> KKQDPPVTHDLRVSLEEIYSGCTKKMKISHKRLNPDGKSIRNEDKILTIEVKKGWKEGTKITFPKEGDQTSNNIPADIV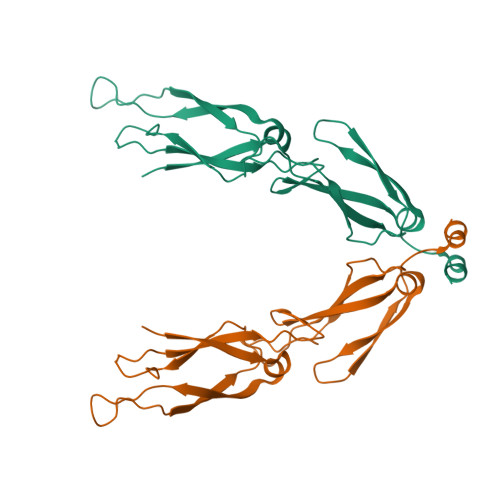FVLKDKPHNIFKRDGSDVIYPARISLREALCGCTVNVPTLDGRTIPVVFKDVIRPGMRRKVPGEGLPLPKTPEKRGDLIIEFEVIFPERIPQTSRTVLEQVLPI> XGEAAAA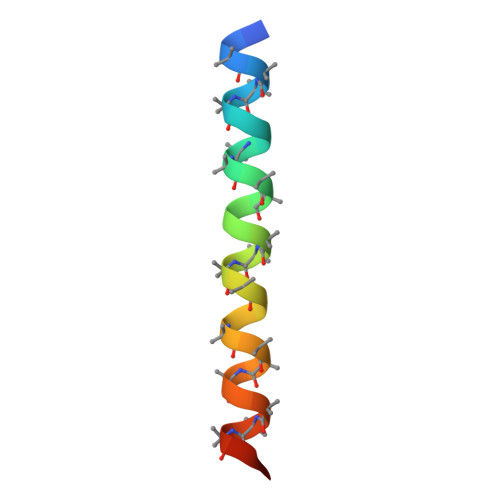KEAAAAKEAAAAKEAAAAKAAAWKGX The capsaicin- and heat-activated receptor, TRPV1, has served as a model for deciphering lipid modulation, which is relevant to understanding how pro-algesic agents enhance channel activity in the setting of inflammatory pain. Identification of a pocket within the TRPV1 transmembrane core has provided initial clues as to how phosphoinositide lipids bind to and regulate the channel. Here we show that this regulatory pocket in rat TRPV1 can accommodate diverse lipid species, including the inflammatory lipid lysophosphatidic acid, whose actions are determined by their specific modes of binding. We captured several states of TRPV1 ranging from channels in which the VBP is empty to those bearing different bioactive lipids, including distinct phosphoinositide species, brominated phosphoinositide analogs and a pro-algesic lipid, lysophosphatidic acid (LPA). Together, our data show how the VBP accommodates a range of bioactive lipids and how occupancy of the site corresponds to the structural status of the pore.

To visualize the lipid–channel complex, we added LPA to nanodisc-reconstituted TRPV1 and determined a consensus cryo-EM map to a resolution of 3.0 Å. Through symmetry expansion and focused classification, we captured LPA bound within the vanilloid pocket in multiple stoichiometries, ranging from apo to all four subunits occupied. With resting and fully liganded structures representing closed and open configurations of the pore (S6) helices, respectively, we examined intermediate conformational states associated with substochiometric LPA binding (the four subunits are denoted as A through D in a counterclockwise orientation as viewed from the extracellular face). However, when the second LPA binds to an adjacent subunit (A and B), we see that gating transitions occur in the S6 helices owing to ejection of the resident PI lipid from both neighboring pockets, which communicate by virtue of domain-swap architecture. Specifically, we see that one S6 helix (S6-A) is in the open configuration and the neighboring helix (S6-B) is in an intermediate position between open and closed because the resident PI lipid in the C subunit prevents full backward movement of S6-B. S6-C and S6-D remain in closed configurations. The binding of the third LPA induces all four S6 helices to adopt the π–α transition, with the S6-B and S6-C in the open configuration and the S6-D and S6-A helices in intermediate positions. Together, these observations are consistent with a model in which ligand binding induces allosteric gating movements in the adjacent VBP through domain-swap interactions. From this analysis, we infer that the first LPA binds to TRPV1 randomly, but such binding increases the affinity for binding to the adjacent versus the opposite monomer.

>[4x]GAMGSRLYDRRSIFDAVAQSNCQELESLLPFLQRSKKRLTDSEFKDPETGKTCLLKAMLNLHNGQNDTIALLLDVARKTDSLKQFVNASYTDSYYKGQTALHIAIERRNMTLVTLLVENGADVQAAANGDFFKKTKGRPGFYFGELPLSLAACTNQLAIVKFLLQNSWQPADISARDSVGNTVLHALVEVADNTVDNTKFVTSMYNEILILGAKLHPTLKLEEITNRKGLTPLALAASSGKIGVLAYILQREIHEPECRHLSRKFTEWAYGPVHSSLYDLSCIDTCEKNSVLEVIAYSSSETPNRHDMLLVEPLNRLLQDKWDRFVKRIFYFNFFVYCLYMIIFTAAAYYRPVEGLPPYKLKNTVGDYFRVTGEILSVSGGVYFFFRGIQYFLQRRPSLKSLFVDSYSEILFFVQSLFMLVSVVLYFSQRKEYVASMVFSLAMGWTNMLYYTRGFQQMGIYAVMIEKMILRDLCRFMFVYLVFLFGFSTAVVTLIEDGKYNSLYSTCLELFKFTIGMGDLEFTENYDFKAVFIILLLAYVILTYILLLNMLIALMGETVNKIAQESKNIWKLQRAITILDTEKSFLKCMRKAFRSGKLLQVGFTPDGKDDYRWCFRVDEVNWTTWNTNVGIINEDPG>[2x]ASQPNSSAKKKEEKGKNIQVVVRCRPFNLAERKASAHSIVECDPVRKEVSVRTGGLADKSSRKTYTFDMVFGASTKQIDVFRSVVCPILDEVIMGYNCTIFAYGQTGTGKTFTMEGERSPNEEYTWEEDPLAGIIPRTLHQIFEKLTDNGTEFSVKVSLLEIYNEELFDLLNPSSDVSERLQMFDDPRNKRGVIIKGLEEITVHNKDEVYQILEKGAAKRTTAATLMNAYSSRSHSV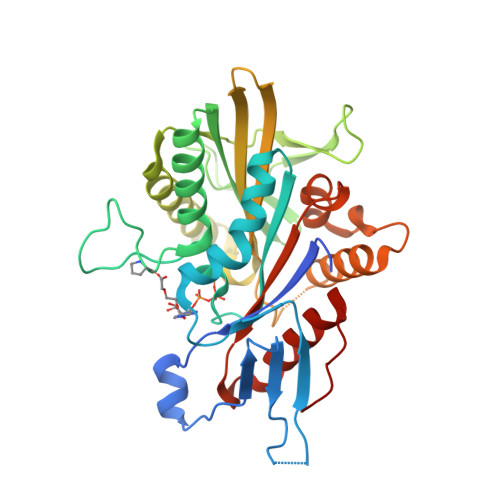FSVTIHMKETTIDGEELVKIGKLNLVDLAGSENIGRSGAVDKRAREAGNINQSLLTLGRVITALVERTPHVPYRESKLTRILQDSLGGRTRTSIIATISPASLNLEETLSTLEYAHRAKNILNKPEVNQK>[2x]MSDKDSKNTPQVPEKLGLSRRGFLGASAVTGAAVAATALGGAVMTRESWAQAVKESKQKIHVGPGELDDYYGFWSGGHQGEVRVLGVPSMRELMRIPVFNVDSATGWGLTNESRHIMGDSAKFLNGDCHHPHISMTDGKYDGKYLFINDKANSRVARIRLDIMKCDKMITVPNVQAIHGLRLQKVPHTKYVFANAEFIIPHPNDGKVFDLQDENSYTMYNAIDAETMEMAFQVIVDGNLDNTDADYTGRFAAATCYNSEKAFDLGGMMRNERDWVVVFDIHAVEAAVKAGDFITLGDSKTPVLDGRKKDGKDSKFTRYVPVPKNPHGCNTSSDGKYFIAAGKLSPTCSMIAIDKLPDLFAGKLADPRDVIVGEPELGLGPLHTTFDGRGNAYTTLFIDSQVVKWNMEEAVRAYKGEKVNYIKQKLDVHYQPGHLHASLCETNEADGKWLVALSKFSKDRFLPVGPLHPENDQLIDISGDEMKLVHDGPTFAEPHDCI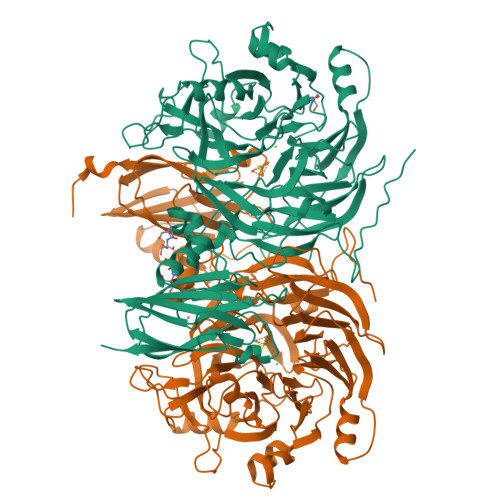MARRDQIKTKKIWDRNDPFFAPTVEMAKKDGINLDTDNKVIRDGNKVRVYMTSMAPAFGVQEFTVKQGDEVTVTITNIDQIEDVSFGFVVVNHGVSMEISPQQTSSITFVADKPGLHWYYCSWFCHALHMEMVGRMMVEPAWSHPQFEK>[8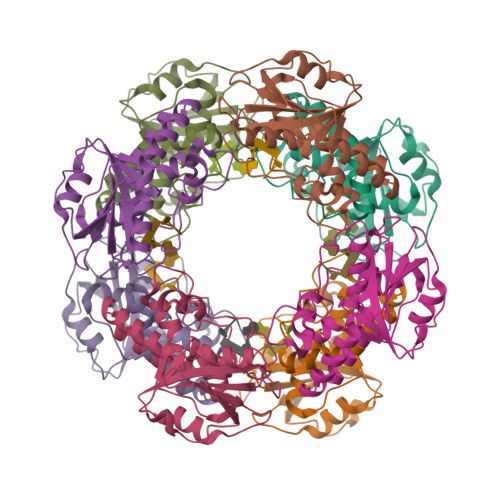x]SMTEIRVHQGDLPNLDNYRIDAVAVDTETLGLQPHRDRLCVVQLSSGDGTADVIQIAKGQKSAPNLVRLLSDRDITKIFHFGRFDLAILAHTFGVMPDVVFCTKIASKLTRTYTDRHGLKEICGELLNVNISKQQQSSDWAAETLSRAQIEYAASDVLYLHRLKDIFEERLKREERESVAKACFQFLPMRANLDLLGWSEIDIFAHS> NRLSVKLPGLDLKNPIIPASG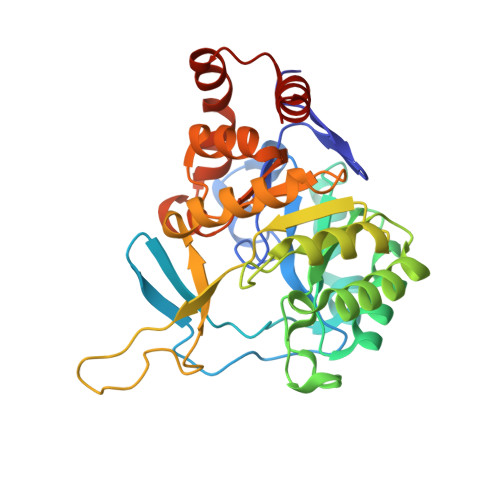CFGFGEEYAKYYDLNKLGSIMVKATTLHPRFGNPTPRVAETASGMLNAIGLQNPGLEVIMAEKLPWLNENFPDLPIIANVAGSEEDDYVAVCAKIGDAPNVKVIELNISCPNVKHGGQAFGTDPDVAAALVKACKAVSKVPLYVKLSPNVTDIVPIAKAVEAAGADGLTMINTLMGVRFDLKTRKPVLANITGGLSGPAIKPVALKLIHQVAQVVDIPIIGMGGVESAQDVLEMYMAGASAVAVGTANFADPFVCPKIIEKLPEVMDQYGIDSLENLIQEVKNSK The high-resolution crystal structure of an Acinetobacter baumannii protein previously reported as being dependent on the type VI secretion system has been determined. The encoded protein, which is classed as a member of the tautomerase superfamily on the basis of sequence homology, represents a putative effector. Structural and sequence comparisons reveal significant conservation with the tautomerase superfamily of enzymes, which are not generally noted as being associated with this secretion system. Members of the tautomerase superfamily form distinctive trimers or hexamers and the crystal structure indicates that AbTFM forms a stable assembly that belongs to the trimer group.

The structure of AbTFM, with a single subunit in the asymmetric unit, was determined by molecular replacement and refined using diffraction data extending to 1.75 Å resolution. The resulting model consists of residues Met1–Leu121. Due to the lack of reliable electron density, the first two residues (Gly-His), which are remnants of the TEV protease cleavage site, and the last eight (Leu-Leu-Asn-Tyr-Gln-Val-Asn-Ile) residues are absent. The compact fold of the AbTFM subunit, in which about 75% of the residues are in elements of secondary structure, displays the characteristic β–α–β repeat structure of the longer tautomerase superfamily. There are three other short β-strands: β3 occurs in the loop linking β2 and β4, and β6 and β7 then form an antiparallel alignment at the C-terminal end of the polypeptide. AbTFM forms a homotrimer exploiting a crystallographic threefold axis of symmetry parallel to c. The interactions between elements of secondary structure on each subunit to form three seven-stranded β-sheets are important for trimer formation. The interface between each monomer creates three identical pockets lined with positively charged side chains. The shape and the charge of these pockets would be consistent with AbTFM binding a small acidic entity. The trimer presents three putative active or binding sites separated by approximately 25 Å. Each site is primarily constructed within a single subunit, with a combination of primarily nonpolar side chains and basic residues, in a relatively small depression formed between the β-sheet and the two helices.

> MSQVKIYANERTIIQYRELLSHAIHQALIEELKYPVEKRFQRFISLKPENFIYPSDRSQHYIIIELSMFAGRSPATKKQLIQTLFRNIEEQCKIAPQDIEITIFETPKENWGIRGKNADELLLNYQVNI>GPPQMSATNEDLKTNFHSLHNQMRQMPMSHFREALDAPDYSGMRQSGFFAMSQGFQLESHGGDVFMHAHRENPQCKG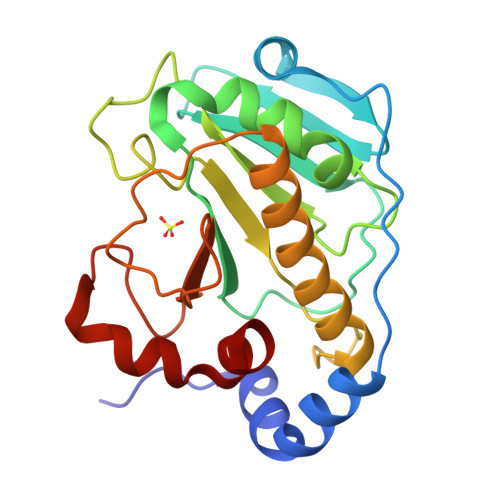DFAGDKFHISVQREQVPQAFQALSGLLFSVDSPIDKWKVTDMERVDQQSRVAVGAQFTLYVKPDQENSQYSASSLHNTRQFIECLESRLSESGLMPGQYPESDVHPENWKYVSYRNELRSGRDGGEMQSQALREEPFYRLMAE[2x]> GPLGSPQCKALYAYDAQDTDELSFNAN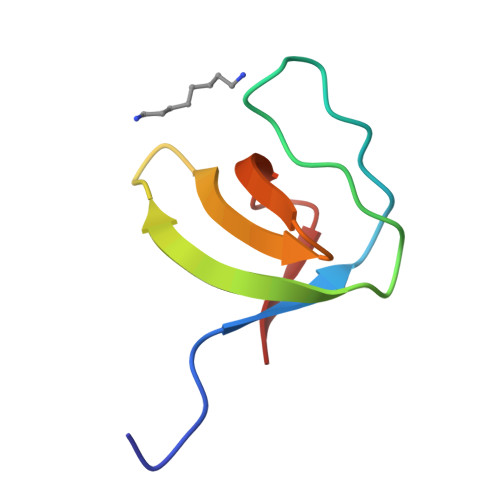DIIDIIKEDPSGWWTGRLRGKQGLFPNNYVTKI> 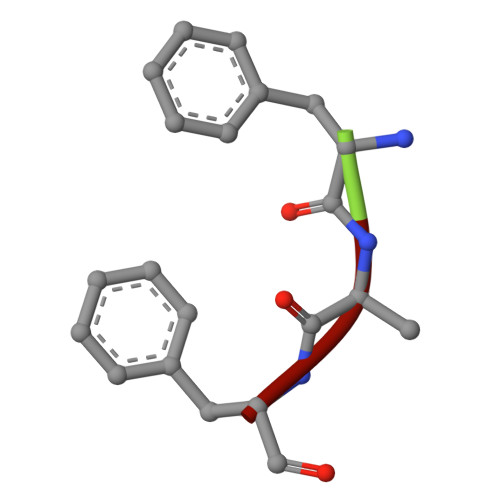FAF> MDAKARNC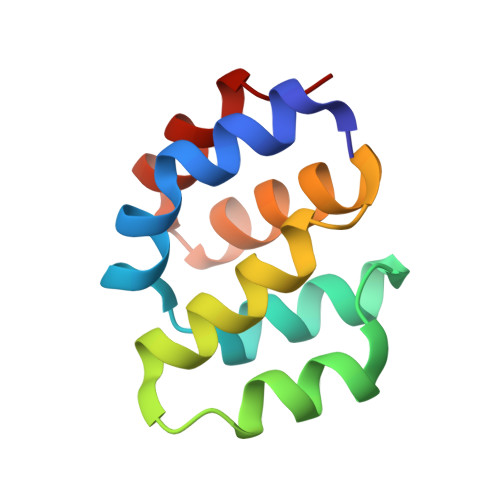LLQHREALEKDIKTSYIMDHMISDGFLTISEEEKVRNEPTQQQRAAMLIKMILKKDNDSYVSFYNALLHEGYKDLAALLHDGIP>GTGDGSTVLTKDRIIEIIERKTGMSREEIEEEIRKIMEEDPYLSEQGAAALLAERLGIDLIEKEEVSLMRISELYPGMDPREVNVVGRVLKKYPPREYTRKDGSVGRVASLIIYDDSGRARVVLWDAKVSEYYNKIEVGDVIKVLDAQVKESLSGLPELHINFRARIILNPDDPRVEMIPPLEEVRVATYTRKKIKDI[2x]

Replication Protein A (RPA) is a heterotrimeric single stranded DNA-binding protein with essential roles in DNA replication, recombination and repair. In Archaea, the same function is also fulfilled by a heterotrimeric RPA. We report three crystal structures and five cryo-EM structures of Pyrococcus abyssi RPA (hereafter referred to PabRPA), in its apo form as well as bound to ssDNA. We find that archaeal and eukaryotic RPAs share a conserved heterotrimerization core, which is composed of three OB domains connected through a three-helix bundle formed by a C-terminal α-helix from each subunit.

To gain insights into the contacts between AROD and OB-1, the crystal structure of the Rpa1 N-terminal domains AROD-OB-1 was determined at 1.8 Å resolution. AROD folds into a three-helix bundle, which is stabilized by a conserved hydrophobic core, and is connected to OB-1 by a 9-aa linker. AROD is an acidic domain, which contains 10 solvent-exposed glutamic acid residues out of 56 residues. The high-resolution view of the AROD-OB-1 interface shows that all three helices of AROD contribute to the interaction with OB-1. The chemical nature of the interactions at the interface is diverse and includes networks of direct and water-mediated buried polar contacts, as well as contacts between hydrophobic residues. Remarkably, the interface includes three salt bridges that involve two acidic residues (E23 and E27) and one basic residue (K17) from AROD. To test the effect of the disruption of this interaction on the DNA-binding properties of OB-1, we compared the binding of wild-type AROD-OB-1 and a triple mutant (K17A-E23A-E27A) to a surface-immobilized poly-dT35 ssDNA by BLI. Strikingly, the AROD-OB-1 triple mutant shows a 10-fold higher affinity for ssDNA than the wild-type construct (KD = 72.0 ± 17.0 nM vs 847 ± 216 nM). Altogether, these results show that interaction with AROD modulates the DNA-binding activity by OB-1. Consistently, the structure reveals that AROD binds next to the DNA-binding site of OB-1, with its solvent-exposed glutamic acid residues pointing toward the DNA-binding cleft.> GPGSPITDERVYESIGQYGGETVKIVRIEKARDIPLGATVRNEMDSVIISRIVKGGAAEKSGLLHEGDEVLEINGIEIRGKDVNEVFDLLSDMHGTLTFVLIPSQQIKPPPAKETVIHVKAHFDYDPSDDPYVPCRELGLSFQKGDILHVISQEDPNWWQAYREGDEDNQPLAGLVPGKEEILTYEEMSLYHQPANRKRPIILIGPQNCGQNELRQRLMNKEKDRFASAVPHTTRSRRDQEVAGRDYHFVSRQAFEADIAAGKFIEHGEFEKNLYGTSIDSVRQVINSGKICLLSLRTQSLKTLRNSDLKPYIIFIAPPSQERLRALLAKEGKNPKPEELREIIE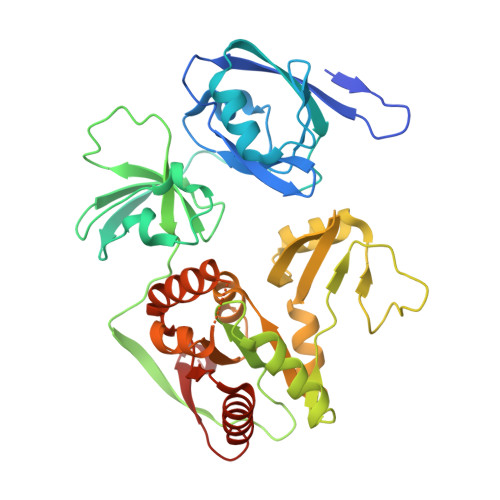KTREMEQNNGHYFDTAIVNSDLDKAYQELLRLINKLDTEPQWVPSTWLR> MNLCNVNNYYLIIAEKSKAAKKIAEALSEKPILCRKYNVSYWIIKDHNSSKYVIVPAAGHLFGLKGESGFPVYDADWKPLWEIDKNSYYTKRYYQLISSLSKYALGFINACDYDIEGSVIGYLIIKNLGDIKKAKRMKFSA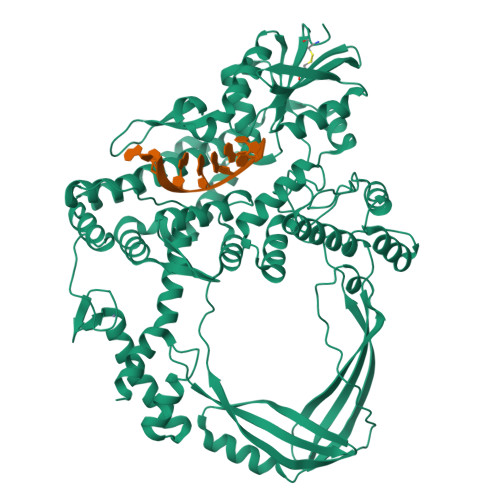LTKSDILSAFRNISALDYDMINAGIARHKIDWLWGINVSRALMISLQDFAKKRVILSAGRVQSPTLVQVVNSEIERNLFIPLPKFTVSIIVKIKDYSLNIKVNKEFEKITEAKEFLNKLINKTVKVVEVENRVRLLERPSPFNLTDLQIEAGRIYGISPYNVERIAEDLYLDGLISFPRTNSQKIPSTISIYNIIKGLENSSYRKLVDLVRKITGGKYVVKQGIKDDPAHPAIHPTGEAPKNLPNSKFKIYDLIARRFLGSVSADAKLSNTIYTLKVSDFPLEFTVSYTKILERNWLDIYHFHNVKEDKPIFLSKGDEGKIVDGKVNISLSKPTSRYTKVSLLKWMESSNLGTEATRGRIIEILVKRKYLTNNGRYIIPTKLGFYIAEILNKFFPDIVDVRMTADMESKLEMIKTGKVLESKVIKENIEKLNKFIEEYKVNKDKVGESLAKALGLIKIVKCKYCDLEQYKDGLCKYHYEAKVRLLDAVEIWKERTKYDHKKILKRISSSKSTGKYVKDIVTYMLSSE> GMANDQDLSNPEYLYTEDDINQLLKHYLGLDDRISIIQHVALNESLLL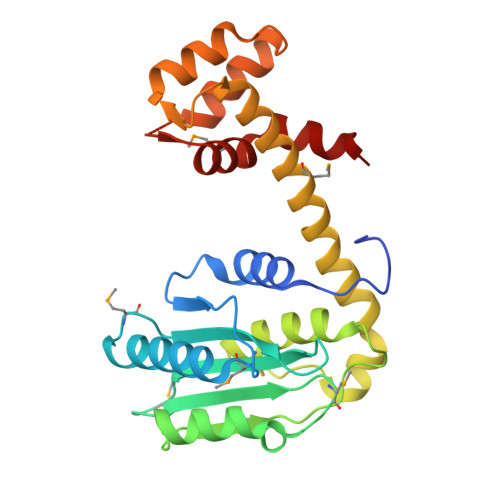KQTLHQVLSDIFSGMQEKAVIPLHTGNNHWVAMAIKKGMNDDIVISYNDPMGVSIDDKVTLINCIKELCPGAKINDLQTVQQTNVYDCGPFVVDNLIKMSQGQPILSTEEAKQQAQNIRQSQVNFLSENRMITSAAAALADTLLKNNNRITEGVLVDRIFDNKILSVQEKQQLLNNLLDNHIKENKSLTKESLTRMLASTHFVQQQANVLLN> MSALPEEVNRTLLQIVQAFASPDNQIRSVAEKALSEEWITENNIEYLLTFLAEQAAFS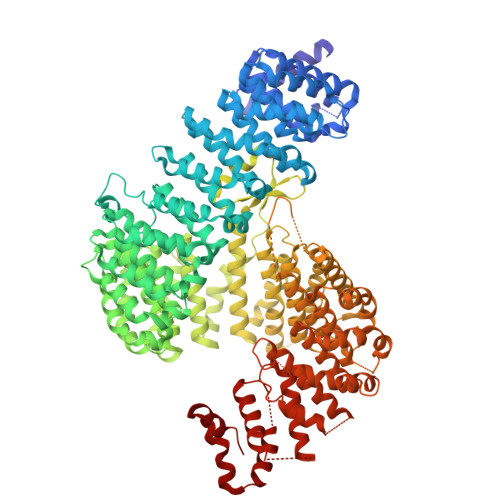QDTTVAALSAVLFRKLALKAPITHIRKEVLAQIRSSLLKGFLSERADSIRHKLSDAIAECVQDDLPAWPELLQALIESLKSGNPNFRESSFRILTTVPYLITAVDINSILPIFQSGFTDASDNVKIAAVTAFVGYFKQLPKSEWSKLGILLPSLLNSLPRFLDDGKDDALASVFESLIELVELAPKLFKDMFDQIIQFTDMVIKNKDLEPPARTTALELLTVFSENAPQMCKSNQNYGQTLVMVTLIMMTEVSIDDDDAAEWIESDDTDDEEEVTYDHARQALKRVALKLGGEYLAAPLFQYLQQMITSTEWRERFAAMMALSSAAKGCADVLIGEIPKILDMVIPLINDPHPRVQYGCCNVLGQISTKFSPFIQRTAHDRILPALISKLTSECTSRVQTHAAAALVNFSEFASKDILEPYLDSLLTNLLVLLQSNKLYVQEQALTTIAFIAEAAKNKFIKYYDTLMPLLLNVLKVNNKDNSVLKGKCMECATLIGFAVGKEKFHEHSQELISILVALQNSDIDEDDALRSYLEQSWSRICRILGDDFVPLLPIVIPPLLITAKATQDVGLIEEEEAANFQQYPDWDVVQVQGKHIAIHTSVLDDKVSAMELLQSYATLLRGQFAVYVKEVMEEIALPSLDFYLHDGVRAAGATLIPILLSCLLAATGTQNEELVLLWHKASSKLIGGLMSEPMPEITQVYHNSLVNGIKVMGDNCLSEDQLAAFTKGVSANLTDTYERMQDRHGDGDEYNENIDEEEDFTDEDLLDEINKSIAAVLKTTNGHYLKNLENIWPMINTFLLDNEPILVIFALVVIGDLIQYGGEQTASMKNAFIPKVTECLISPDARIRQAASYIIGVCAQYAPSTYADVCIPTLDTLVQIVDFPGSKLEENRSSTENASAAIAKILYAYNSNIPNVDTYTANWFKTLPTITDKEAASFNYQFLSQLIENNSPIVCAQSNISAVVDSVIQALNERSLTEREGQTVISSVKKLLGFLPSSDAMAIFNRYPADIMEKVHKWFA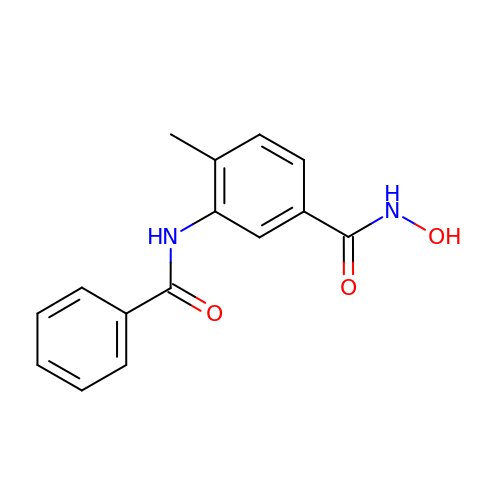3-benzamido-4-methyl-~{N}-oxidanyl-benzamide | C15 H14 N2 O3 | ROYNQMDXPFEFHJ-UHFFFAOYSA-N>[2x]MHTLYAP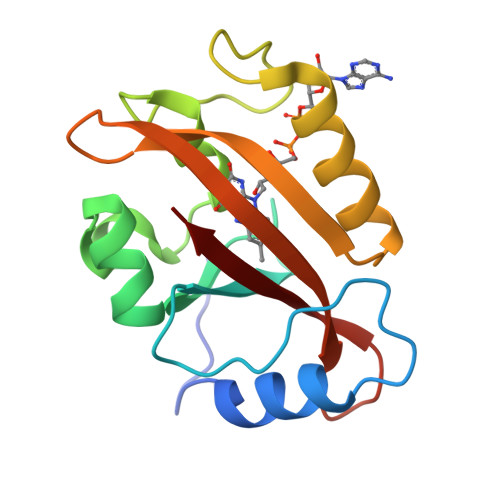GGYDIMGYLIQIMNRPNPQVELGPVDTSSALILCDLKQKDTPIVYASEAFLYMTGYSNAEVLGRNCRFLQSPDGMVKPKSTRKYVDSNTINTMRKAIDRNAEVQVEVVNFKKNGQRFVNFLTMIPVRDETGEYRYSMGFQCE>[16x]MVRFLDGH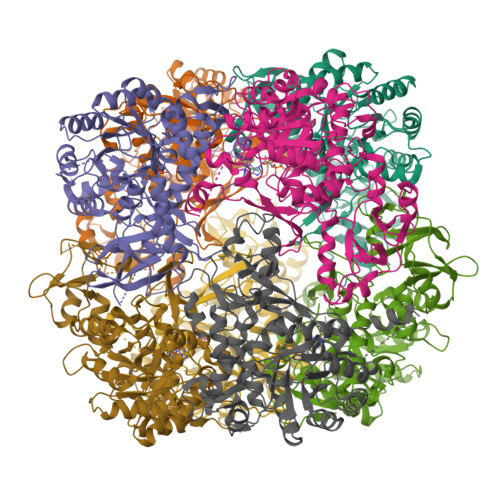TPAYDLTYNDVFVVPGRSDVASRFDVDLSTVDGSGTTIPVVVANMTAVAGRRMAETVARRGGIVVLPQDLPITAVSETVDFVKSRDLVVDTPVTLSPEDSVSDANALLHKRAHGAAVVVFEGRPIGLVTEANCAGVDRFARVRDIALSDFVTAPVGTDPREVFDLLEHAPIDVAVMTAPDGTLAGVLTRTGAIRAGIYTPAVDAKGRLRIAAAVGINGDVGAKAQALAEAGADLLVIDTAHGHQAKMLDAIKAVASLDLGLPLVAGNVVSAEGTRDLIEAGASIVKVGVGPGAMCTTRMMTGVGRPQFSAVVECAAAARQLGGHVWADGGVRHPRDVALALAAGASNVMIGSWFAGTYESPGDLLFDRDDRPYKESYGMASKRAVAARTAGDSSFDRARKGLFEEGISTSRMSLDPARGGVEDLLDHITSGVRSTCTYVGAANLPELHEKVVLGVQSAAGFAEGHPLPAGWTAAAKEDLEHHHHHHHH> AASGSALIFDEEMSRYKLLWTDPECEIEVPERLTVSYEALRTHGLAQRCKAVPVRQATEQEILLAHSEEYLEAVKQTPGMNVEELMAFSKKYNAVYFHQNIYHCAKLAAGATLQLVDSVMKREVRNGMALVRPPGHHSQRSAANGFCVFNNVAFAALYAKKNYNLNRILIVDWDVHHGQGIQYCFEEDPSVLYFSWHRYEHQSFWPNLPESDYSSVGKGKGSGFNINLPWNKVGMTNSDYLAAFFHVLLPVAYEFDPELVIVSAGFDSAIGDPEGEMCALPEIFAHLTHLLMPLAAGKMCVVLEGGYNLTSLGQSVCQTVHSLLGDPTPRISGLGTACDSALESIQNVRNVQSSYWSSFKHLAQSENNPKRPRLDATNGGPKESSEPASESNPKKTAQDIVWPEPLKRMPASVRTVVVPPPGVELTLPKNCQHSGDISESTAKEVQRIRDKHFHDLTDQNILRSLGNIISVLDRMMRSDEVCNGCVVVSDLSVSVQCALQHALTEPAERVLVVYVGDGELPVKTNDGKVFLVQICTKETEDKCVNRLTLCLREGESLTAGFMQALLGLILPVAYEFNPALVLGIVEETAAKTRLMRVWGHMTCLIQGLARGRMLTLLQGYDKDLLELTVSALSG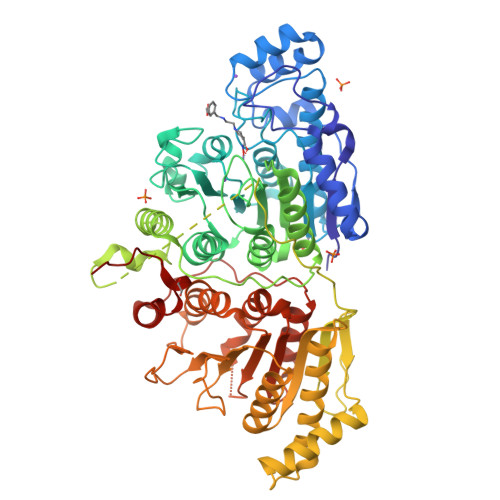ASISPLGPLRAPKPEDVEMMEKQRQRLQERWGLLRCTVSESW>[4x]MGHHHHHHSHMSNPIQAEVLKRVAEVFDQHVPFHNLLGLDIKRYDIDGVEVAINMKPELIGNIHQQILHGGVTATVL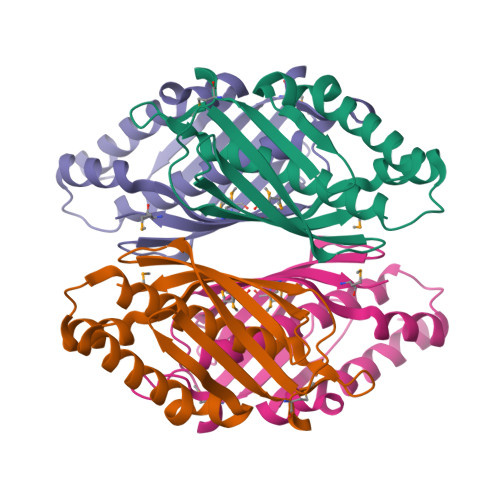DVVGGLTAFAGLVASRDDWTIEELQQRLQTLGTIDMRVDYLRPGRGQIFTGTGSVIRAGNRVSVCRMELHNEQGTHIAFGTGTYMVG>[2x]GSETLVRPKPELLKLLKSVGAQKDTYTMKEVLFYLG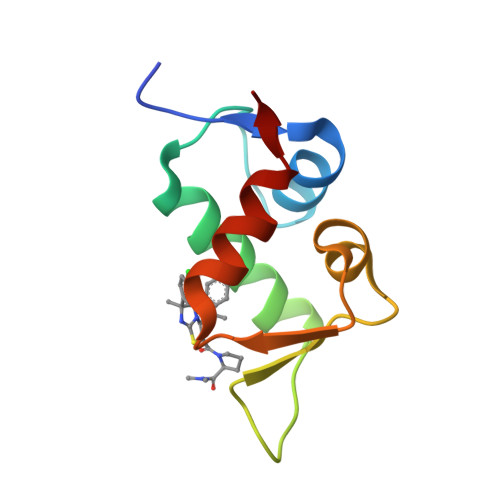QYIMTKRLYDEKQQHIVYCSNDLLGDLFGVPSFSVKEHRKIYTMIYRNLVV> SNAMSEAEAKLWQ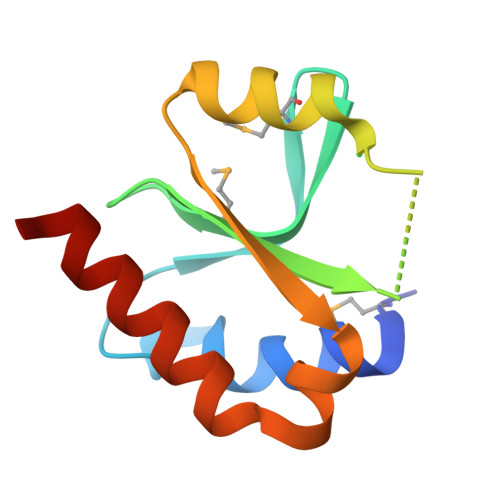HLRAGRLNGYKFRRQQPMGNYIVDFMCVTPKLIVEADGGQHAEQAVYDHARTVYLNSLGFTVLRFWNHEILQQTNDVLAEILRVLQELEKQ2-(3-BENZOYLPHENOXY)ETHYL(HYDROXY)FORMAMIDE | C16 H15 N O4 | 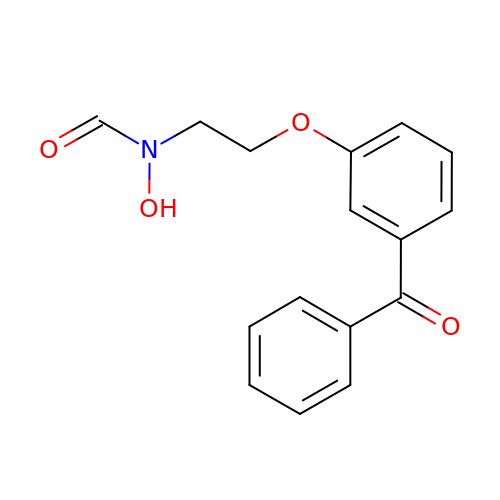ZHFKBNAHHTUQBH-UHFFFAOYSA-N>[2x]MMAGPLSGLRVVELAGIGPGPHAAMILGDLGADVVRIDRPSSVDGISRDAMLRNRRIVTADLKSDQGLELALKLIAKADVLIEGYRPGVTERLGLGPEECAKVNDRLIYARMTGWGQTGPRSQQAGADINYISLNGILH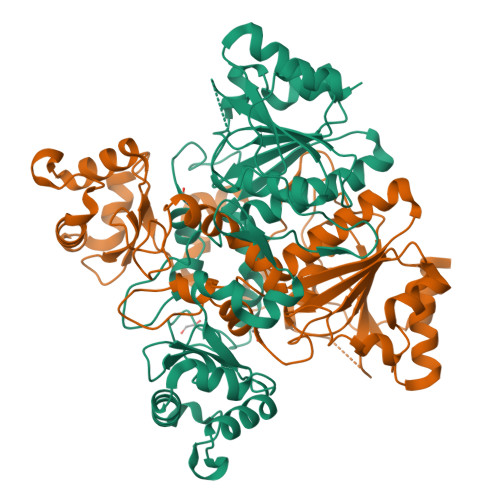AIGRGDERPVPPLNLVGDFGGGSMFLLVGILAALWERQSSGKGQVVDAAMVDGSSVLIQMMWAMRATGMWTDTRGANMLDGGAPYYDTYECADGRYVAVGAIEPQFYAAMLAGLGLDAAELPPQNDRARWPELRALLTEAFASHDRDHWGAVFANSDACVTPVLAFGEVHNEPHIIERNTFYEANGGWQPMPAPRFSRTASSQPRPPAATIDIEAVLTDWDGGSGC Herein, we have chosen to use an extracellular dye-type heme peroxidase found in Streptomyces lividans and referred to as DtpAa. The overall structure reveals a ferredoxin-like fold typical of dye decolourizing peroxidases with two DtpAa monomers in the crystallographic asymmetric unit. Heme enzymes catalyse many essential reactions in biology and understanding their structures throughout their reaction cycles is of high interest, prompting extensive efforts made to obtain ‘intact’ structures at high resolution. A major challenge is to obtain the higher valence states of these proteins, for example peroxidases (FeIII resting state and FeIV intermediate states), as these states are phenomenally sensitive to reduction in synchrotron experiments caused by the presence of large numbers of solvated electrons or other radiolytically produced species, generated by the interaction of X-rays with the crystal.

To produce an ‘anchor’ structure of DtpAa, i.e. resting state ferric, free of any effects of the X-ray beam on the structure, we used the SACLA XFEL beamline BL2 EH3 to perform SFX with an X-ray energy of 10 keV, a pulse length of 10 fs with a 1.25 × 1.34 µm beam and a pulse energy of 289 µJ pulse−1. The chip was translated between apertures in the 33 ms separating the 30 Hz XFEL pulses, with a single image recorded at each position. The SFX structure was determined to a resolution of 1.88 Å from a total of 72 615 indexed and merged diffraction patterns [Fig. 2(a), Table S1]. The refined model exhibited a mean-determined B factor of 34.7 Å2. The heme Fe is six-coordinate with residue His326 acting as the proximal ligand with an Fe—N bond length of 2.19 Å (we note here that monomer B appears to be inactive and is consequently not discussed further). The distal heme coordination site is occupied by a well defined, full occupancy water molecule (W1), bound to the Fe at a distance of 2.40 Å. A number of further, well defined water molecules occupy the remainder of the heme distal pocket [Fig. 2(a)]. W1 is hydrogen bonded to a second water, W2, at a distance of 2.68 Å and also interacts with the charged side chains of Asp239 (2.92 Å) and Arg342 (2.74 Å). Interestingly, the side chains of these two amino acids are only 3.13 Å apart (Arg Nη1 to Asp Oδ2) suggesting a charge-based interaction. A linear fit to the data yields an intercept (i.e. extrapolated to zero dose) of 2.37 Å, which is very close to the value in the SFX structure (2.40 Å) at comparable resolution and within the experimental error for this bond length in the room-temperature structures.

>[2x]DPAGADAGSAVPFHGAHQAGIATPVQDRLHFAAFDVTTEDRAAFVALLKEWTAAARRLTAGHAVGEGAYGGLPEAPPDDTGEALGLKPSRLTLTIGFGPSLFTRFGLADLRPEALADLPKFPGDNLDRARSGGDLCVQACADDPQVAVHAIRNLARIGFGKVVVRWSQLGFGKTSSTTPDKQTPRNLLGFKDGTRNIAGTEKDRLDRFVWAAEKDGTPWMTGGSYLVARRIRMHIETWDRASLQEQEDVFGRDKGEGAPVGKAKERDEPFLKAMKPDAHVRLAHPDSNGGATLLRRGYSFTDGTDGLGRLDAGLFFLAYQRDIRTGFVPVQRNLATDALNEYIQHVGSAVFAVPPGVRDADDWWGSTLFGKEA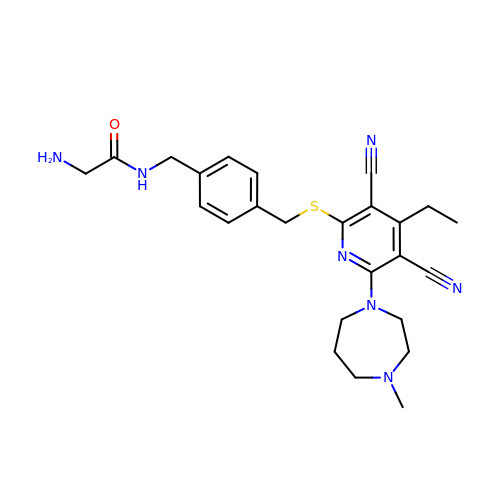N-{[4-({[3,5-dicyano-4-ethyl-6-(4-methyl-1,4-diazepan-1-yl)pyridin-2-yl]sulfanyl}methyl)phenyl]methyl}glycinamide | C25 H31 N7 O S | QPLFMVVUDGWTPG-UHFFFAOYSA-N> GAMSANGKISVPEAVVNWLFKVIQPIYNDGRTTFHDSLALLDNFHSLRPRTRVFTHSDGTPQLLLSIYGTISTGEDGSSPHSIPVIMWVPSMYPVKPPFISINLENFDMNTISSSLPIQEY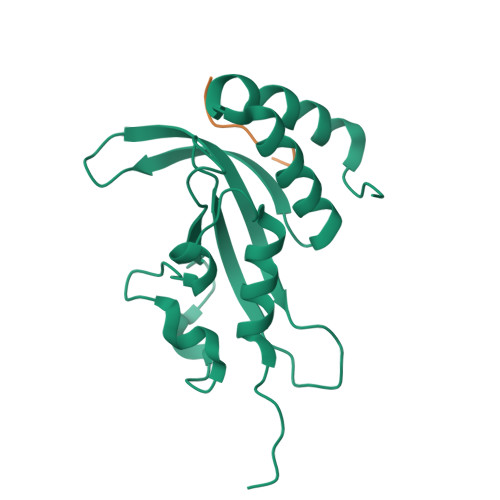IDSNGWIALPILHAWDPAAMNLIMVVQELMSLLHEPPQDQA;> QVPSDPYNY> GYTRERTNRHFFVSRANAFFSRLPISRIQRALA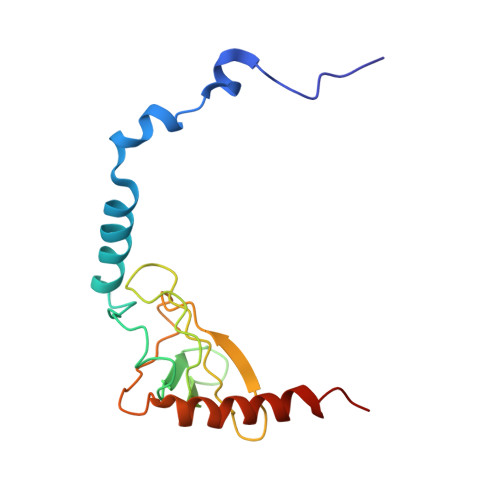MEAIKKGSMKPWKHTKEQIIGSPITCNFEYNPRPVRLIGTVMDAHTEETSIKGGLKVYARSEEANMMLWIPAGNPKLKYEVTAAKGSFEHYLDERSKWDEAWLTGRARMK>[8x]KQNAPWNFQSKVVTDTLFSKVLNSKRAYTVFLPKSFEQNKEKKYPVLYLLHGMWETNPVWAERGHVKDVMDRLVASGEACEMIIVTPNAGGNIHLEWNGYFDMPGWKYETFFYTEFLPYIEKKYRVIGDRQHRAIAGLSMGGGGATNYGQRHSDMFCAVYAMSALMSIPEQGAVPADDPNSKIAILTRSVIENSCVKYVMEADEDRKADLRSVAWFVDCGDDDFLLDRNIEFYQAM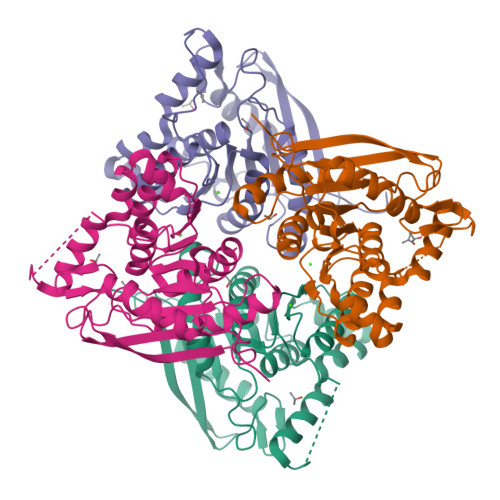RNAGVPCQFRVRDGGHDWEYWHSALYQCLPFVTRIFGKE>SLFELGKMILQETGKNPAKSYGAYGCNCGVLGRGKPKDATDRCCYVHKCCYKKLTGCNPKKDRYSYSWKDKTIVCGEN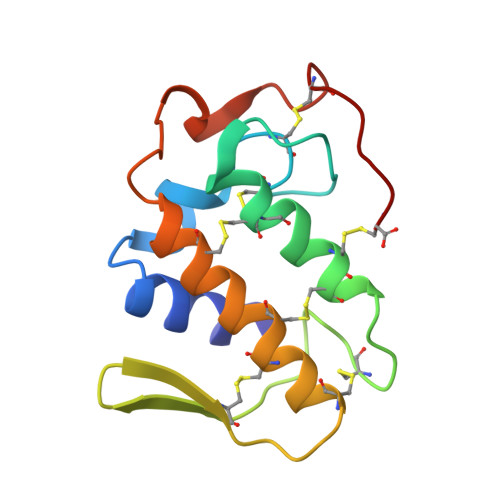NSCLKELCECDKAVAICLRENLNTYNKKYRYYLKPLCKKADAC[2x]> MAPQGPPIPVLGGWQKKTPVDNEQYKELAHFAVSKQVEGREFFDTVLEVTDVET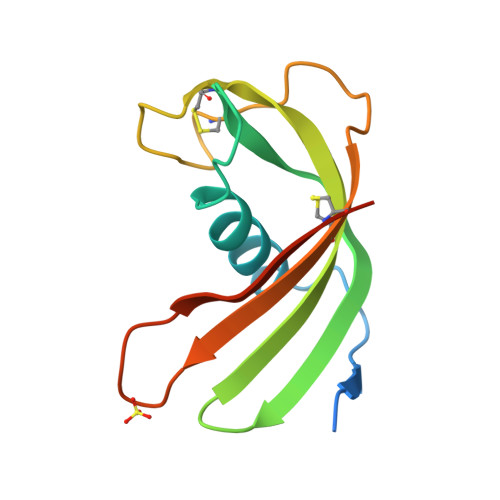QVVAGTNYRITFKIAESTCRVTETYSKETCLPKTRDVKSTCTAVITEPLNNERFVHSFTCGGAAASK>[2x]AVLLLGEVTNGALNRDATAKAVAAVKALGDVTVLCAGASAKAAAEEAAKIAGVAKVLVAEDALYGHRLAEPTAALIVGLAGDYSHIAAPATTDAKNVMPRVAALLDVMVLSDVSAILDADTFERPIYAGNAIQVVKSKDAKKVFTIRTASFDAAGEGGTAPVTET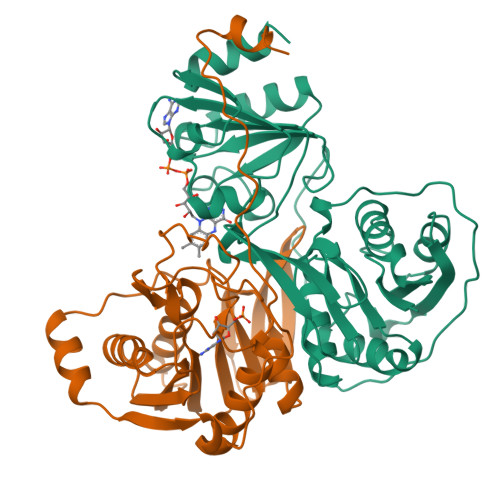AAAADPGLSSWVADEVAESDRPELTSARRVVSGGRGLGSKESFAIIEELADKLGAAVGASRAAVDSGYAPNDWQVGQTGKVVAPELYVAVGISGAIQHLAGMKDSKVIVAINKDEEAPIFQIADYGLVGDLFSVVPELTGKL;>[2x]MKVLVPVKRLIDYNVKARVKSDGSGVDLANVKMSMNPFDEIAVEEAIRLKEKGQAEEIIAVSIGVKQAAETLRTALAMGADRAILVVAADDVQQDIEPLAVAKILAAVARAEGTELIIAGKQAIDNDMNATGQMLAAILGWAQATFASKVEIEGAKAKVTREVDGGLQTIAVSLPAVVTADLRLNEPRYASLPNIMKAKKKPLDEKTAADYGVDVAPRLEVVSVREPEGRKAGIKVGSVDELVGKLKEAGVI2-(5-methylsulfonylpyridin-3-yl)-1,1-bis(oxidanylidene)-4-[[2,4,6-tris(fluoranyl)phenyl]methyl]pyrido[2,3-e][1,2,4]thiadiazin-3-one 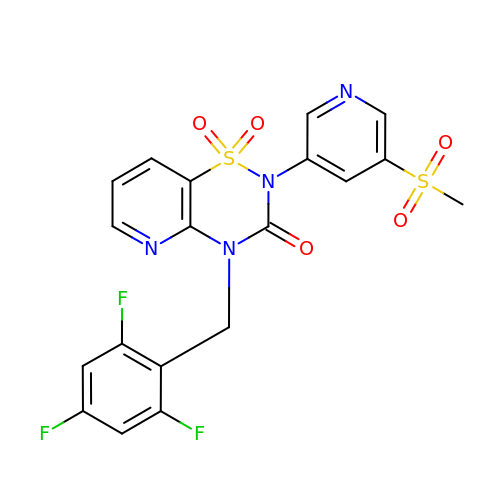| C19 H13 F3 N4 O5 S2 | LWKUASRJTUZHSJ-UHFFFAOYSA-N>[2x]MAIEFNIQESKILKGVYIITPNKFRDLRGEI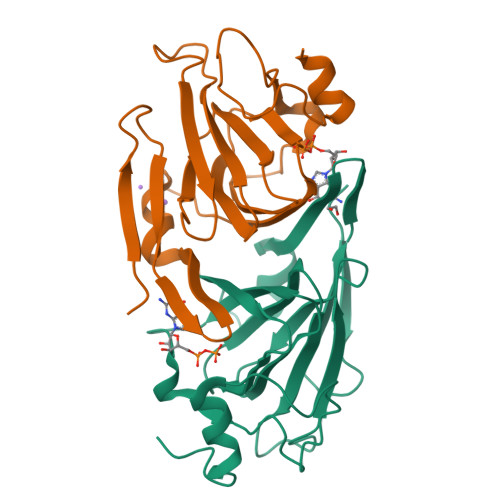WTAFTSKAVDKLLPNGLKFIHDKFIHSKHNVIRGIHGDVKTYKLATCVYGEIHQVVVDCRKDSPTYLKYEKFIINQDNQQIILVPAGFGNAHYVTSESAVYYYKCAYKGDYVDAPDQFTYAWNDERIGIDWPTNSPILSERDILATKNKGLEHHHHHH> VDWTDAERAAIKALWGKIDV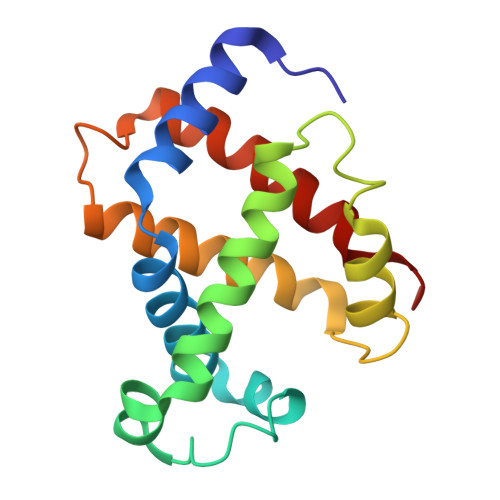GEIGPQALSRLLIVYPWTQRHFKGFGNISTNAAILGNAKVAEHGKTVMGGLDRAVQNMDNIKNVYKQLSIKHSEKIHVDPDNFRLLGEIITMCVGAKFGPSAFTPEIHEAWQKFLAVVVSALGRQYH>[4x]MKKNLFLSIIFSFCVILQAFASDTVFVRETQIPVLIERQDNVLFMLRLNAKESHTLDEVVLNFGKDVNMSDIQSVKLYYSGTEARQNYGKNFFAPVSYISSHTPGKTLAANPSYSINKSQVNNPKRKVALKANQKLFPGINYFWISLQMKPDASLLDKVAAKIAAIKVDNKEALM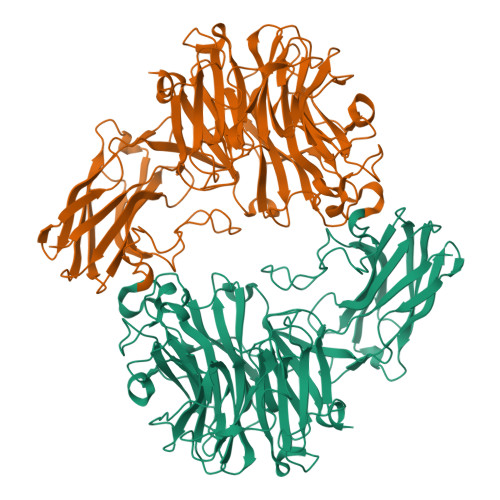HTVSPENIVHRVGVGVRHAGDDGSASFRIPGLVTTNKGTLLGVYDVRYNNSADLQEHVDIGLSRSVDGGKTWEKMRLPLAFGETGDLPAAQNGVGDPSILVDTKTNTVWVVAAWTHGMGNQRAWWSSYPGMDMNHTAQLVLSKSTDDGKTWSKPINITEQVKDPSWYFLLQGPGRGITMQDGTLVFPIQFIDSTRVPNAGIMYSKDRGETWKIHNYARTNTTEAQVAEVEPGVLMLNMRDNRGGSRAISTTKDLGKTWTEHSSSRKALQEPVCMASLISVKAKDNVLNKDILLFSNPNTVKGRHHITIKASLDGGVTWLPEHQVMLDEGEGWGYSCLTMIDKETIGILYESSVAHMTFQAVQLRDIIKHHHHHHHHHH> ACHPRLSLHRPALEDLLLGSEANLTCTLTGLRDASGVTFTWTPSSGKSAVQGPPERDLCGCYSVSSVLPGCAEPWNHGKTFTCTAAYPESKTPLTATLSKSGNTFRPEVHLLPPPSEELALNELVTLTCLARGFSPKDVLVRWLQGSQELPREKYLTWASRQEPSQGTTTFAVTSI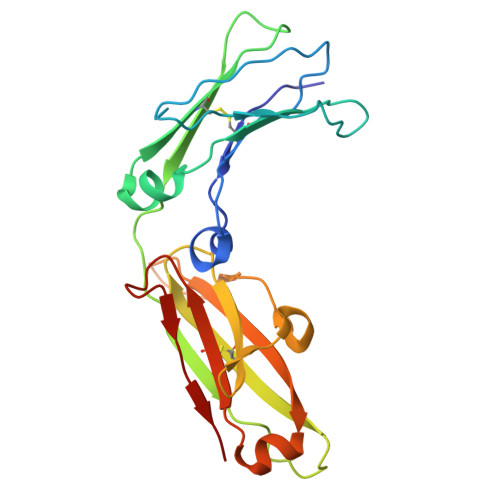LRVAAEDWKKGDTFSCMVGHEALPLAFTQKTIDRLAGK>MKKHIIIKTIPKKEEIISRDLCDCIYYYDNSVICKPIGPSKVYVSTSLENLEKCLQLHYFKKLVKNIEIFDEVHNSKPNCDKCLIVEIGGVYFVRRVNGVPR[2x]

Recently, genomic evidence has implicated a critical role for disulfide bonds in the structural stabilization of intracellular proteins from certain of these organisms, contrary to the conventional view that structural disulfide bonds are exclusively extracellular. Considering the apparent abundance of disulfide bonding in P. aerophilum, proteins containing multiple cysteines in their amino acid sequences would be expected to have a high likelihood of containing disulfide bonds. To test this, a 98-residue protein containing six cysteine residues was selected from the P. aerophilum genome for structural characterization. The protein (GI 18312142) could not be assigned a function or three-dimensional fold in advance, as it had no recognizable sequence similarity to proteins of known function or structure.

The crystal structure of the protein was determined to a resolution of 1.6 Å with an R-factor of 18.4%. The first 70 amino acid residues constitute an N-terminal domain whose three-dimensional fold has been observed previously in the copper chaperone Atx1, but which does not contain the active-site residues of Atx1. The remaining 18 residues form a small C-terminal domain of novel fold that interacts with the N-terminal domain exclusively through hydrophobic contacts. The three-dimensional structure reveals that the six cysteine residues in the primary sequence are paired to form three disulfide bonds in the native fold (C22–C34, C24–C54, and C80–C83). Although one disulfide bond (C80–C83) fits the sequence of a potential metal-binding/active-site CxxC motif, the C22–C34 and C24–C54 disulfide bonds do not fit any known metal-binding or active-site motifs and appear to serve structural roles within the protein fold. Of the 16 P. aerophilum proteins whose structures have been determined to date, a total of 29 cysteine residues have been visualized, and 23 of these have been found to form disulfide bonds. Despite the still relatively small sample size, these numbers provide important three-dimensional structural support for the claim of abundant disulfide bonds in this organism, meriting a further survey of thermophilic protein structures. In every case where more than one cysteine is present within a P. aerophilum protein of known structure, a disulfide bond is found. As expected, Pyrobaculum aerophilum, an organism singled out in earlier studies, exhibits a high propensity for cysteines to be in close proximity, with pairs of cysteine residues appearing in proximity nearly ten times more often than expected by chance. Some organisms have evidently modulated their internal biochemistry to enable disulfide bonding as a key mechanism for stabilizing their proteins at high temperatures.(8S)-3',8-cyclo-7,8-dihydroguanosine 5'-triphosphate 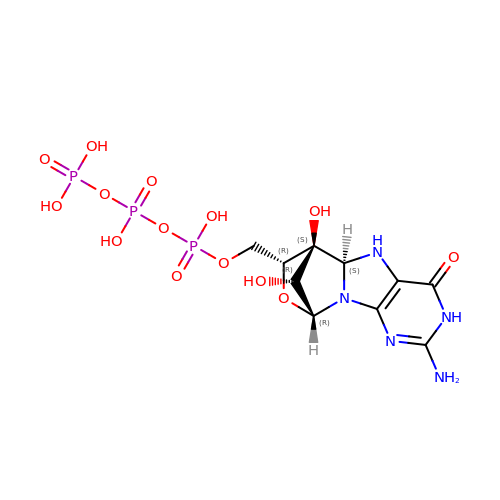| C10 H16 N5 O14 P3 | HRBCPXBJAWPPIC-FKPGNCNUSA-N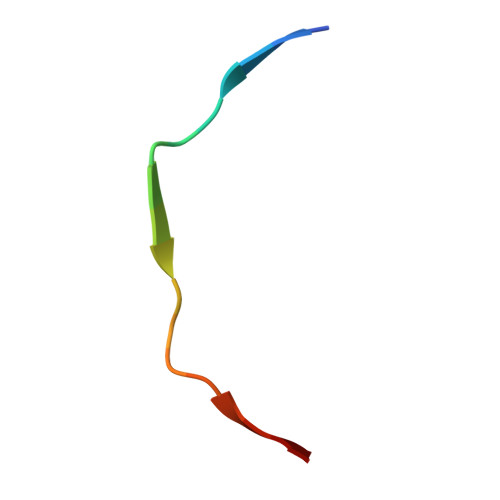> NAHNFPLDLASAESAPVA> SAPILQSLLSCSRAAATDPGLAAAELASVRAAATDAGDPSERLAFYFADALSRRLACGTGAPPSAEPDARFASDELTLCYKTLNDACPYSKFAHLTANQAILEATGAATKIHIVDFGIVQGIQWAALLQALATRPEGKPTRIRITGVPSPLLGPQPAASLAATNTRLRDFAKLLGVDFEFVPLLRPVHELNKSDFL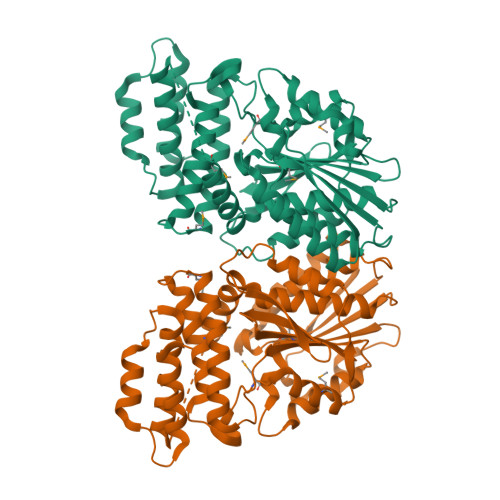VEPDEAVAVNFMLQLYHLLGDSDELVRRVLRLAKSLSPAVVTLGEYEVSLNRAGFVDRFANALSYYRSLFESLDVAMTRDSPERVRVERWMFGERIQRAVGPEEGADRTERMAGSSEWQTLMEWCGFEPVPLSNYARSQADLLLWNYDSKYKYSLVELPPAFLSLAWEKRPLLTVSAWR> PISPIETVPVKLKPGMDGPKVKQWPLTEEKIKALVEICTEMEKEGKISKIGPENPYNTPVFAIKKKDSTKWRKLVDFRELNKRTQDFWEVQLGIPHPAGLKKKKSVTVLDVGDAYFSVPLDEDFRKYTAFTIPSINNETPGIRYQYNVLPQGWKGSPAIFQSSMTKILEPFKKQNPDIVIYQYMDDLYVGSDLEIGQHRTKIE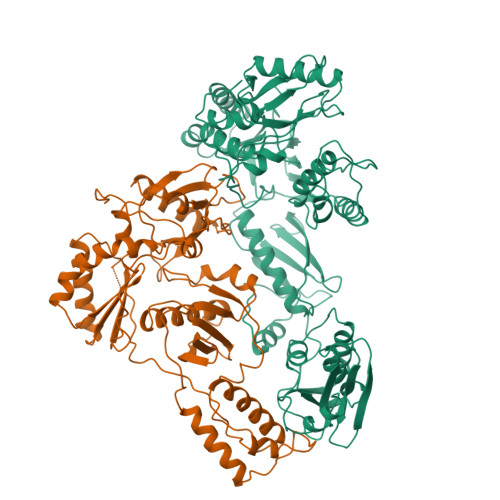ELRQHLLRWGLTTPDKKHQKEPPFLWMGYELHPDKWTVQPIVLPEKDSWTVNDIQKLVGKLNWASQIYPGIKVRQLSKLLRGTKALTEVIPLTEEAELELAENREILKEPVHGVYYDPSKDLIAEIQKQGQGQWTYQIYQEPFKNLKTGKYARMRGAHTNDVKQLTEAVQKITTESIVIWGKTPKFKLPIQKETWETWWTEYWQATWIPEWEFVNTPPLVKLWYQLEKEPIVGAETFYVDGAANRETKLGKAGYVTNKGRQKVVPLTNTTNQKTELQAIYLALQDSGLEVNIVTDSQYALGIIQAQPDKSESELVNQIIEQLIKKEKVYLAWVPAHKGIGGNEQVDKLVSAGI;> PISPIETVPVKLKPGMDGPKVKQWPLTEEKIKALVEICTEMEKEGKISKIGPENPYNTPVFAIKKKDSTKWRKLVDFRELNKRTQDFWEVQLGIPHPAGLKKKKSVTVLDVGDAYFSVPLDEDFRKYTAFTIPSINNETPGIRYQYNVLPQGWKGSPAIFQSSMTKILEPFKKQNPDIVIYQYMDDLYVGSDLEIGQHRTKIEELRQHLLRWGLTTPDKKHQKEPPFLWMGYELHPDKWTVQPIVLPEKDSWTVNDIQKLVGKLNWASQIYPGIKVRQLSKLLRGTKALTEVIPLTEEAELELAENREILKEPVHGVYYDPSKDLIAEIQKQGQGQWTYQIYQEPFKNLKTGKYARMRGAHTNDVKQLTEAVQKITTESIVIWGKTPKFKLPIQKETWETWWTEYWQATWIPEWEFVNTPPLVKLWY>[24x]SSQIRQNYSTEVEAAVNRLVNLYLRASYTYLSLGFYFDRDDVAL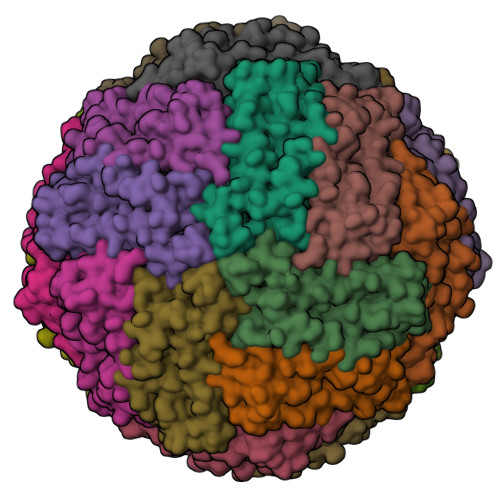EGVCHFFRELAEEKREGAERLLKMQNQRGGRALFQDLQKPSQDEWGTTLDAMKAAIVLEKSLNQALLDLHALGSAQADPHLCDFLESHFLDEEVKLIKKMGDHLTNIQRLVGSQAGLGEYLFERLTLKHD>[2x]MGSSHHHHHHSQDLEVLFQGPHMERPSQENGIQKHRTSLPAPMFSRSDFSVWTILKKCVGLELSKITMPIAFNEPLSFLQRITEYMEHVYLIHRASCQPQPLERMQSVAAFAVSAVASQWERTGKPFNPLLGETYELIREDLGFRFISEQVSHHPPISAF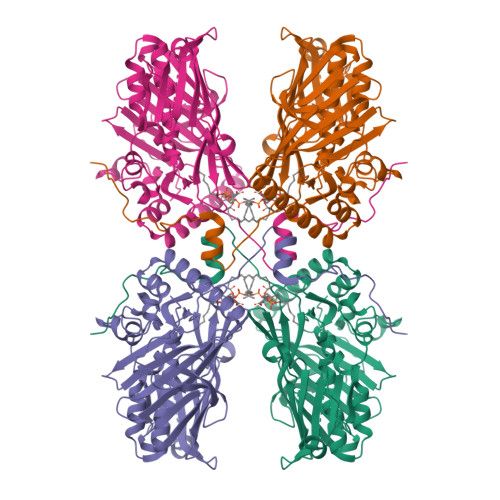HSEGLNHDFLFHGSIYPKLKFWGKSVEAEPRGTITLELLKHNEAYTWTNPTCCVHNVIIGKLWIEQYGTVEILNHRTGHKCVLHFKPCGLFGKELHKVEGHIQDKNKKKLFMIYGKWTECLWGIDPVSYESFKKQERRGDHLRKAKLDEDSGKADSDVADDVPVAQETVQVIPGSKLLWRINTRPPNSAQMYNFTSFTVSLNELETGMEKTLPPTDCRLRPDIRGMENGNMDLASQEKERLEEKQREARRERAKEEAEWQTRWFYPGNNPYTGTPDWLYAGDYFERNFSDCPDIY> GQEEGEDNGGEDNKKLRGALSSAILSEKPNVKWEDVAGLEGAKEALKEAVILPVKFPHLFKGNRKPTSGILLYGPPGTGKSYLAKAVATEANSTFFSVSSSDLVSKWMGESEKLVKQLFAMARENKPSIIFIDEVDALTGTRGEGESEASRRIKTELLVQMNGVGNDSQGVLVLGATNIPWQLDSAIRRRFERRIYIPLPDLAARTTMFEINVGDTPCVLTKEDYRTLGAMTEGYSGSDIAVVVKDALMQPIRKIQSATHFKDVSTEDDETRKLTPCSPG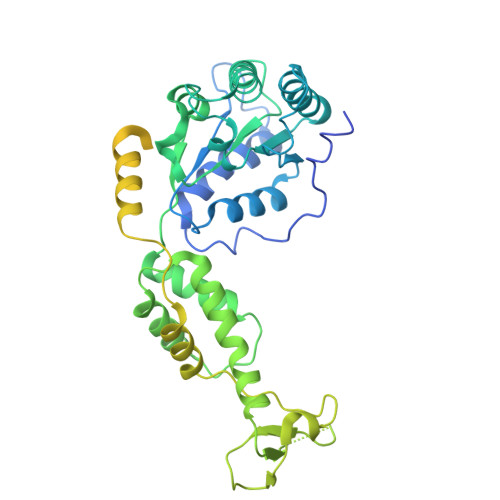DDGAIEMSWTDIEADELKEPDLTIKDFLKAIKSTRPTVNEDDLLKQEQFTRDFGQEGNGGGGSGGGGSGGGGSGGGMAVDMFIKIGDVKGESKDKTHAEEIDVLAWSWGMSQSGSMHMGGGGGAGKVNVQDLSFTKYIDKSTPNLMMACSSGKHYPQAKLTIRKAGGENQVEYLIITLKEVLVSSVSTGGSGGEDRLTENVTLNFAQVQVDYQPQKADGAKDGGPVKYGWNIRQNVQAG>MVASSSLRFDLKSYLKERQRQVEAALNAILPPQDPPLIYESMRYSLLAEGKRLRPILCLASCELAGGTAAIALPTACALEMVHTMSLIHDDLPSMDNDDFRRGRPTNHKVYGEDIAILAGDALLTYAFEAIARHTPEVPADRVLKVIAALARAVGAEGLVGGQVVDLQSEGRDDVN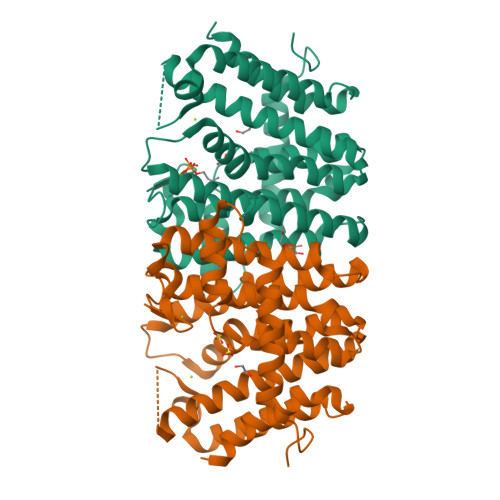LETLHYIHTHKTGALLEVSVVSGAILAGASEELQEQLRTYAQKIGLAFQVIDDILDITATAEELGKTAGKDLAAKKATYPSLLGLDASREYADQLITEAKAAIAAFGAEADPLRAIADYITARKHLLEHHHHHH[2x]> NVSFPASVQLHTAVEMHHWCIPFSVDGQPAPSLRWLFNGSVLNETSFIFTEFLEPAANETVRHGCLRLNQPTHVNNGNYTLLAANPFGQASASIMAAFMDNP;> GFF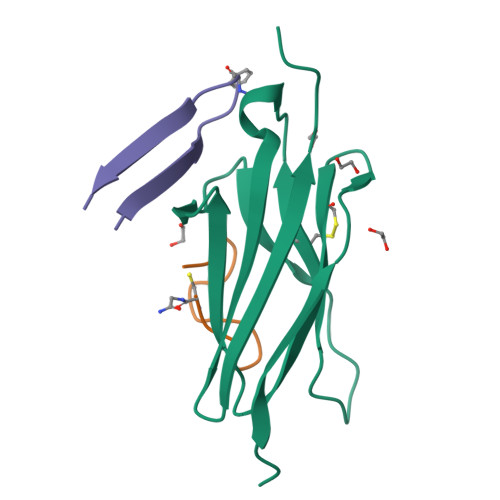LYPHGFYGIVCX;> FKSVSYWGFGRLSYYNHC2-{[2-(morpholin-4-yl)ethyl]amino}-1H-benzimidazole-6-carbohydrazide 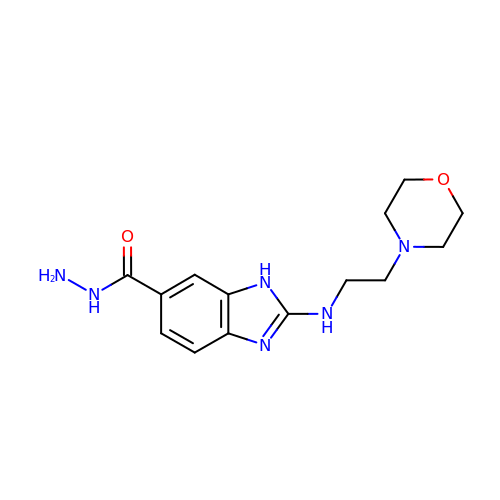| C14 H20 N6 O2 | IGHUHXQGMJQAFS-UHFFFAOYSA-N> RRTLWTTPDTSPNCKMSTEKDSKLTLTLTKCGSQVLGNVSLLAVTGEYHQMTATTKKDVKISLLFDENGILLPSSS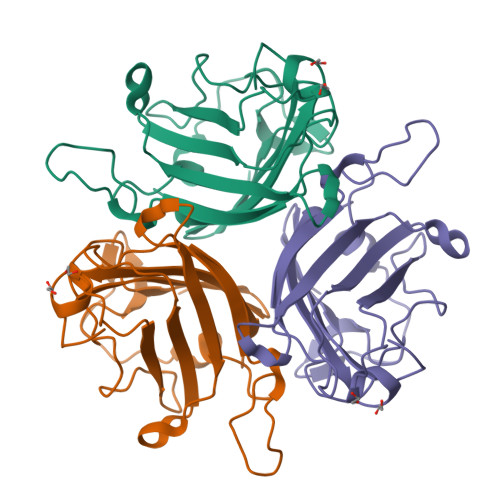LSKDYWNYRSDDSIVSQKYNNAVPFMPNLTAYPKPSAQNAKNYSRTKIISNVYLGALTYQPVIITIAFNQETENGCAYSITFTFTWQKDYSAQQFDVTSFTFSYLTQE> MESKVVVPAQGKKITLQNGKLNVPENPIIPYIEGDGIGVDVTPAMLKVVDAAVEKAYKGERKISWMEIYTGEKSTQVYGQDVWLPAETLDLIREYRVAIKGPLTTPVGGGIRSLNVALRQELDLYICLRPVRYYQGTPSPVKHPELTDMVIFRENSEDIYAGIEWKADSADAEKVIKFLREEMGVKKIRFPEHCGIGIKPCSEEGTKRLVRAAIEYAIANDRDSVTLVHKGNIMKFTEGAFKDWGYQLAREEFGGELIDGGPWLKVKNPNTGKEIVIKDVIADAFLQQILLRPAEYDVIACMNLNGDYISDALAAQVGGIGIAPGANIGDECALFEATHGTAPKYAGQDKVNPGSIILSAEMMLRHMGWTEAADLIVKGMEGAINAKTVTYDFERLMDGAKLLK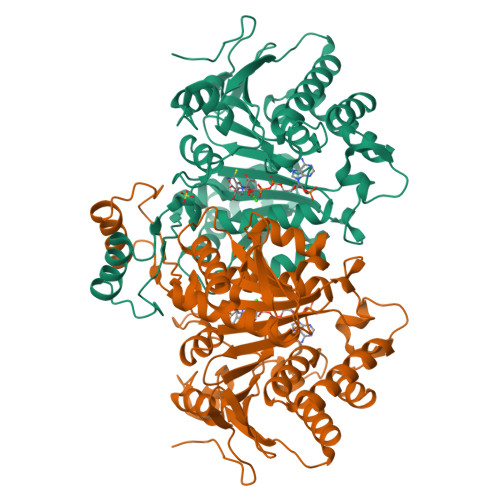CSEFGDAIIENM>[10x]GGMELYLDTADIVAIKRLAKVLPISGVTTNPSIVAKSGK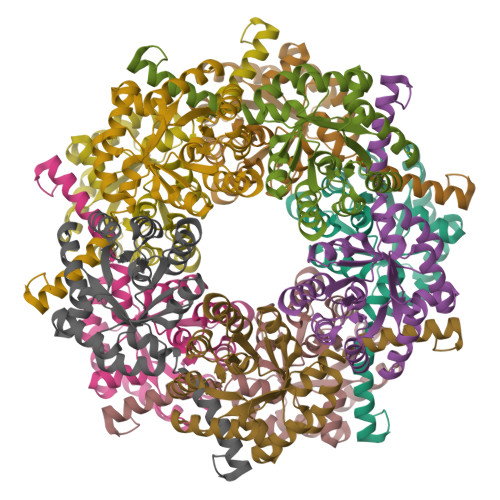PIFLLLNELQEVLGSDKLLFAQVLSSNADEMIKETYQLRKAVPSIVTKIPVNAQGLIAIKELTQQGIPTLGTAVYGAGQGFLAALAGAKYIAPYVNRIDAQGGNSKDTVLELQKLLDLHCPQSLVLAASFRTPRQALDCILAGCKSITLPVDVAELFISDPAVDAVITKFDQDWCNAFGTLSF>MLNQELELSLNMAFARAREHRHEFMTVEHLLLALLSNPSAREALEACSVDLVALRQELEAFIEQTTPVLPASEEERDTQPTLSFQRVLQRAVFHVQSSGRNEVTGANVLVAIFSEQESQAAYLLRKHEVSRLDVVNFISHGTRKDEPTQSSDPGSQPNSEEQAGGEERMENFTTNLNQLARVGGIDPLIGREKELERAIQVLCRRRKNNPLLVGESGVGKTAIAEGLAWRIVQGDVPEVMADCTIYSLDIGSLLAGTKYRGDFEKRFKALLKQLEQDTNSILFIDEIHTIIGAGAASGGQVDAANLIKPLLSSGKIRVIGSTTYQEFSNIFEKDRALARRFQKIDITEPSIEETVQIINGLKPKYEAHHDVRYTAKAVRAAVELAVKYINDRHLPDKAIDVIDEAGARARLMPVSKRKKTVNVADIESVVARIARIPEKSVSQSDRDTLKNLGDRLKMLVFGQDKAIEALTEAIKMARAGLGHEHKPVGSFLFAGPTGVGKTEVTVQLSKALGIELLRFDMSEYMERHTVSRLIGAPPGYVGFDQGGLLTDAVIKHPHAVLLLDEIEKAHPDVFNILLQVMDNGTLTDNNGRKADFRNVVLVMTTNAGVRETERKSIGLIHQDNSTDAMEEIKKIFTPEFRNRLDNIIWFDHLSTDVIHQVVDKFIVELQVQLDQKGVSLEVSQEARNWLAEKGYDRAMGARPMARVIQDNLKKPLANELLFGSLVDGGQVTVALDKEKNELTYGFQSAQKHKAEAAH[6x];>[14x]MSYSGERDNFAPHMALVPMVIEQTSRGERSFDIYSRLLKERVIFLTGQVEDHMANLIVAQMLFLEAENPEKDIYLYINSPGGVITAGMSIYDTMQFIKPDVSTICMGQAASMGAFLLTAGAKGKRFCLPNSRVMIHQPLGGYQGQATDIEIHAREILKVKGRMNELMALHTGQ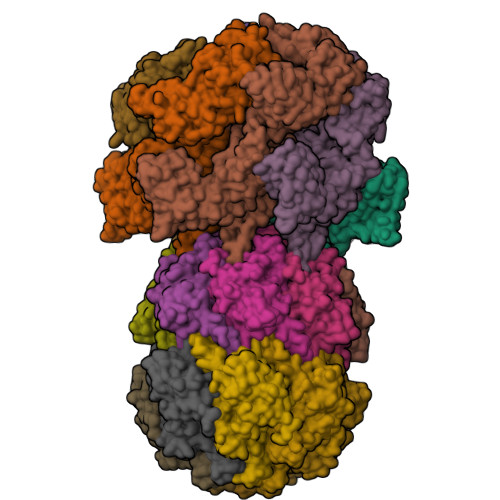SLEQIERDTERDRFLSAPEAVEYGLVDSILTHRN>[3x]LSCGQRLRKSLSSMTRVVGGLVALRGAHPYIAALYWGHSFCAGSLIAPCWVLTAAHCLQDRPAPEDLTVV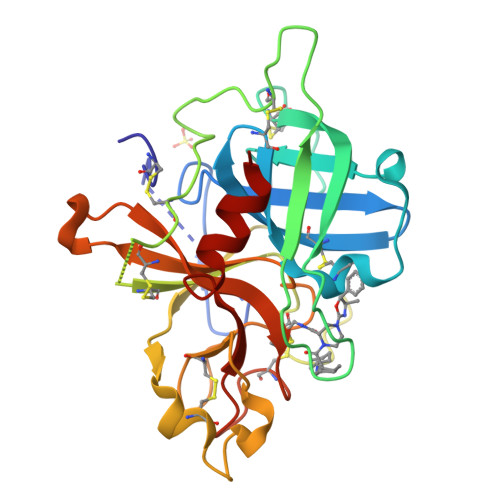LGQERRNHSCEPCQTLAVRSYRLHEAFSPVSYQHDLALLRLQEDADGSCALLSPYVQPVCLPSGAARPSETTLCQVAGWGHQFEGAEEYASFLQEAQVPFLSLERCSAPDVHGSSILPGMLCAGFLEGGTDACQGDSGGPLVCEDQAAERRLTLQGIISWGSGCGDRNKPGVYTDVAYYLAWIREHTVS>[5x]MPVLLGIPLLLRFLGFLLVTLFGYLLTFLKKGFGKIAIAISLFLALIIGLNSILVGYLSDISAQLPSDFVQGV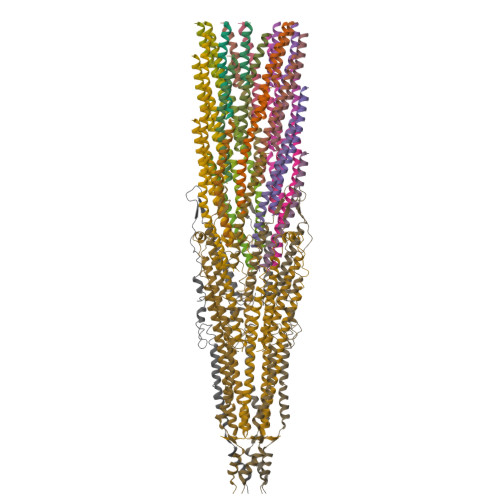QLILPSNALPCFYVILSVKAAIFIFDVKQKIVSYLDWDK;>[5x]AETVESCLAKPHTENSFTNVWKDDKTLDRYANYEGCLWNATGVVVCTGDETQCYGTWVPIGLAIPENEGGGSEGGGSEGGGSEGGGTKPPEYGDTPIPGYTYINPLDGTYPPGTEQNPANPNPSLEESQPLNTFMFQNNRFRNRQGALTVYTGTVTQGTDPVKTYYQYTPVSSKAMYDAYWNGKFRDCAFHSGFNEDPFVCEYQGQSSDLPQPPVNAGGGSGGGSGGGSEGGGSEGGGSEGGGSEGGGSGGGSGSGDFDYEKMANANKGAMTENADENALQSDAKGKLDSVATDYGAAIDGFIGDVSGLANGNGATGDFAGSNSQMAQVGDGDNSPLMNNFRQYLPSLPQSVECRPFVFGAGKPYEFSIDCDKINLFRGVFAFLLYVATFMYVFSTFANILRNKES;>[35x]AEGDDPAKAAFDSLQASATEMIGYAWAMVVVIVGATIGIKLFKKFTSKAS Noradrenaline | C8 H12 N O3 | 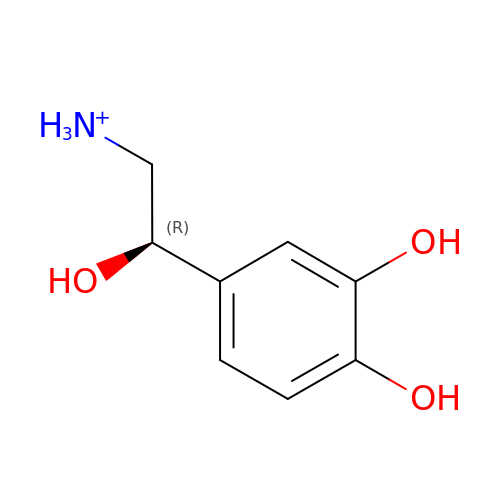SFLSHLFXELFNJZ-QMMMGPOBSA-O>SIDEVGALSKFAASLADQMRAGSNSLDRDVQSLFGVWKGSAADAYRSGWDEMQDGATKVWNALTDIASTLGSNAAAFHAQETSTASSITSTQAD[6x];>[6x]MAAHVESEFSFDLDHIEQVTSRARGFKEFVTENLDQLESRAQKL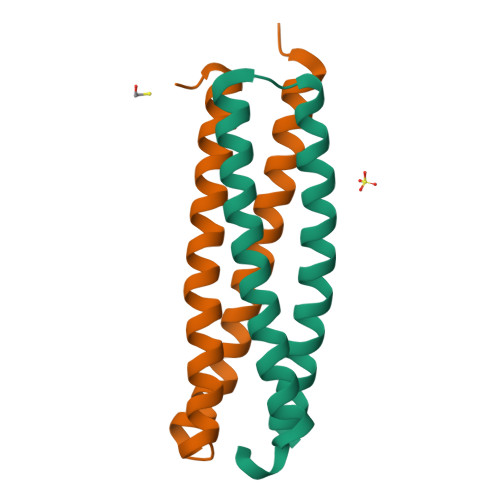VQSGQWAGAAAAAYSQAHKEWMDAARELVEGLSQMEEAARTAHGAYSEAQEANLRMARG>[2x]MSEITLGRFFFERLHQLQVDTVFGLPGDFNLALLDKIYEVDGMRWAGNANELNAGYAADGYARVNPNGLAALVSTFGVGELSLTNAIAGSYSEHVGIINLVGVPSSSAQAKQLLLHHTLGNGDFTVFHRMFKNISQTSAFISDPNTAASEIDRCIRDAYVYQRPVYIGLPSNLVDVKVPKSLLDKKIDLSLHPNEPESQAEVVETVEKFISEASNPVILVDACAIRHNCLKEVAELIAETQFPVFTTPMGKSSVDESNPRFGGVYVGSLSSPDVKEAVESADLVLSVGAMLSDFNTGAFSYNYKTRNVVEFHSDYTKIRQATFPGVQMKEALQVLLKTVKKSVNPKYVPAPVPATKAITTPGNNDPVSQEYLWRKVSDWFQEGDVIISETGTSAFGIVQSKFPKNAIGISQVL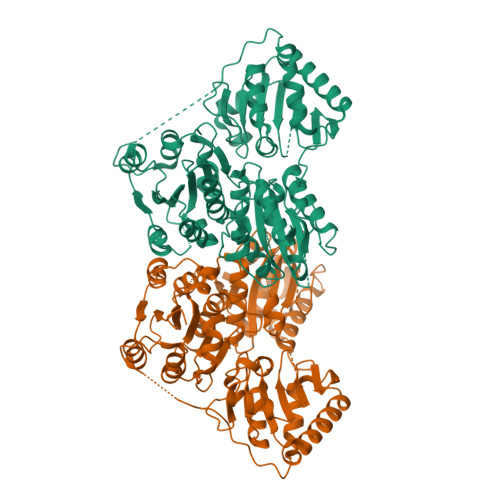WGSIGYATGATCGAAMAAQEIDPKKRVILFTGDGSLQLTVQEISTMCKWDCYNTYLYVLNNDGYTIERLIHGEKAQYNDIQPWNNLQLLPLFNAKKYETKRISTVGELNDLFTNKEFAVPDRIRMVEIMLPVMDAPANLVAQAKQSAATNAAQE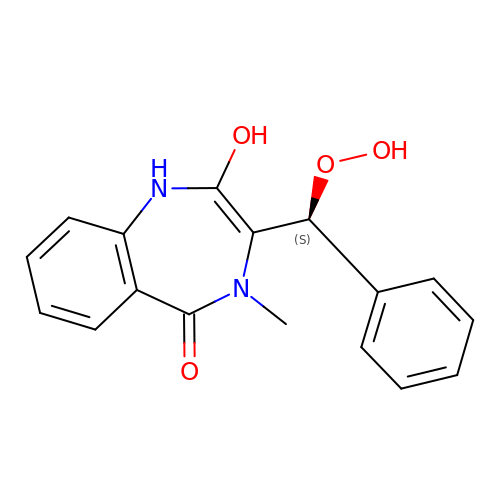3-[(S)-dioxidanyl(phenyl)methyl]-4-methyl-2-oxidanyl-1H-1,4-benzodiazepin-5-one | C17 H16 N2 O4 | UBACWKZQZWEXFD-HNNXBMFYSA-N> FVLTPGNPRWENTHLTYRIENYTPDLSREDVDRAIEKAFQLWSNVSPLTFTKVSEGQADIMISFVRGDHRDNSPFDGPGGNLAHAFQPGPGIGGDAHFDEDERWTKNFRDYNLYRVAAHELGHSLGLSHSTDIGALMYPNYIYTGDVQLSQDDIDGI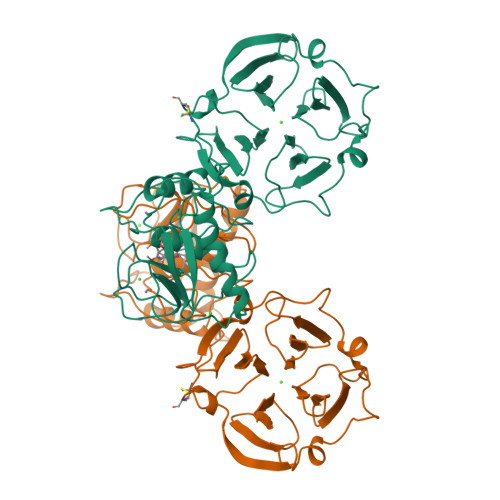QAIYGPSENPVQPSGPQTPQVCDSKLTFDAITTLRGELMFFKDRFYMRTNSFYPEVELNFISVFWPQVPNGLQAAYEIADRDEVRFFKGNKYWAVRGQDVLYGYPKDIHRSFGFPSTVKNIDAAVFEEDTGKTYFFVAHECWRYDEYKQSMDTGYPKMIAEEFPGIGNKVDAVFQKDGFLYFFHGTRQYQFDFKTKRILTLQKANSWFNCRKN>MSLPGNNSAKGTATGNATALWRNAQLATLNPAMDGIGAVENAVIAVRNGRIAFAGPESDLPDDLSTADETTDCGGRWITPALIDCHTHLVFGGNRAMEFEMRLNGATYEEIAKAGGGIVSSVRDTRALSDEVLVAQALPRLDTLLSEGVSTIEIKSGYGLDIETELKMLRVARRLETLRPVRIVTSYLAAHATPADYKGRNADYITDVVLPGLEKAHAEGLADAVDGFCEGIAFSVKEIDRVFAAAQQRGLPVKLHAEQLSNLGGAELAASYNALSADHLEYLDETGAKALAKAG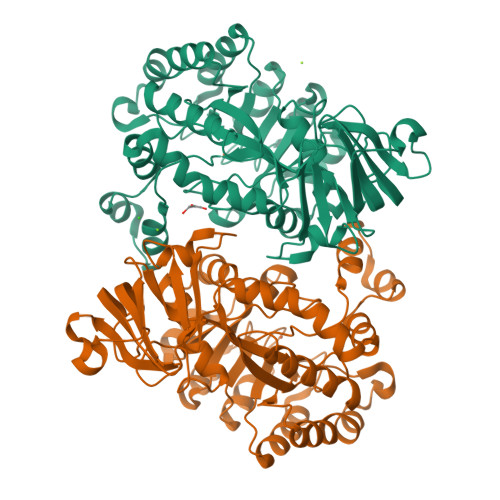TVAVLLPGAFYALREKQLPPVQALRDAGAEIALATDCNPGTSPLTSLLLTMNMGATLFRMTVEECLTATTRNAAKALGLLAETGTLEAGKSADFAIWDIERPAELVYRIGFNPLHARIFKGQKVSPEGHHHHHH[2x]>MGSDKIHHHHHHMKVKKWVTQDFPMVEESATVRECLHRMRQYQTNECIVKDREGHFRGVVNKEDLLDLDLDSSVFNKVSLPDFFVHEEDNITHALLLFLEHQEPYLPVVDEEMRLKGAVSLHDFLEALIEALAMDVPGIRFSVLLEDK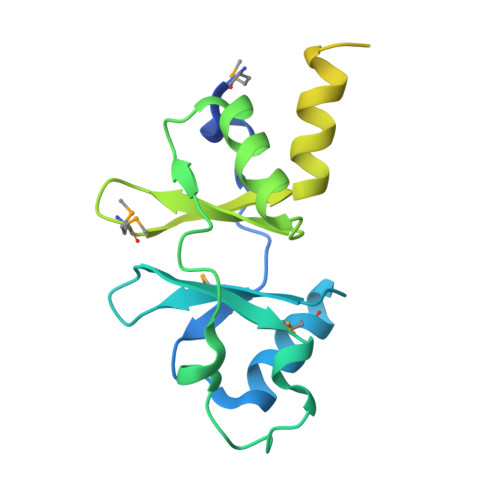PGELRKVVDALALSNINILSVITTRSGDGKREVLIKVDAVDEGTLIKLFESLGIKIESIEKEEGF[2x]>MKLSGVELRRVQMPLVAPFRTSFGTQSVRELLLLRAVTPAGEGWGECVTMAGPLYSSEYNDGAEHVLRHYLIPALLAAEDITAAKVTPLLAKFKGHRMAKGALEMAVLDAELRAHERSFAAELGSVRDSVPCGVSVGIMDTIPQLLDVVGGYLDEGYVRIKLKIEPGWDVEPVRAVRERFGDDVLLQVDANTAYTLGDAPQLARLDP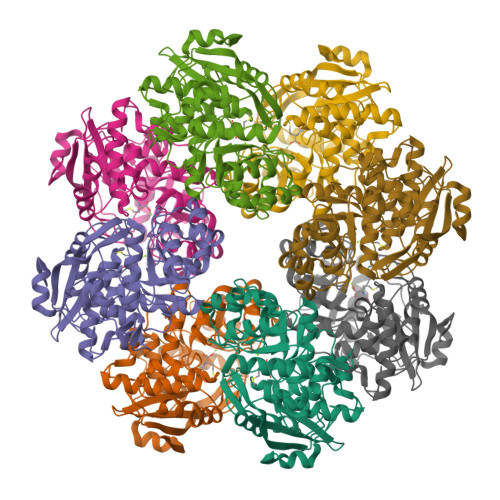FGLLLIEQPLEEEDVLGHAELARRIQTPICLDESIVSARAAADAIKLGAVQIVNIKPGRVGGYLEARRVHDVCAAHGIPVWCGGMIETGLGRAANVALASLPNFTLPGDTSASDRFYKTDITEPFVLSGGHLPVPTGPGLGVAPIPELLDEVTTAKVWIGS[4x]> MPSATPGAPAASAAMQEALEGAGRIIDRLLQEDRAYPDLSELLNVPVHTCPTISGVSEMDYPLQSPGLLTIPSLPEISAIRRVPLPPELIEQFGHMQCNCMMGVFPEISRAWLTIDSDIFMWNYEDGGDLAYYDGLSETILSVGLVKPKTGIFQPHIRFLLVLSTPVDIVILGLSFANLQPGNLNDSISGGMQLLPDPLYSLPTDNTYLLSITSTDNGRIFLSGKDGCLYEVEYQAEAGWFSQRCRKINHSKSSLSFLVPSVLQFAFSEDDPIVQIAIDNSRNILYTRSEKGVIQVYDLGVDGHGMSRVASVSQNSLVSAAGNIARTIDRNVFKPIIHISVIEMSESVNCHLLAVTHTGVRFYFSTVPFKQPTARPCMLALVHVRLPPGFSASSNVEKPSKVHKALYNNGVLLMAASENEDNDMLWCINRDSFPFQKPMMETQVTTQVDGHSWALSAVDEQKADKIVTPLNKDLIPLTDSPVIIQQHMIPPKRFVLLSAQGSHIFYKLRPVDQLRHLLVSNSGGDGEEIERFFKLHQENQACATCLILACSSAASDREVSSWAARAFFRYGGEAQLRVQSALHAPSNVGPIFGSPLPVASPIPVGSPMPNPSFLGTPTQGACPPNVSTPAYGVATPAPQPPAVPGMMGTEIVFSGKHNGICIYFCRIIGNIWDGSVAVENTFQSGNREVTAIDSSVTPQHLESVLKELKGLLEFLDRYSQFTAGSLGNPGFGTPANRQQRLVSLGRPDIGSSQQAQQELQRKYHTEAQLAEQFSLQGIHQLVRKMCQALALWKLLCEHQFSLVVSDLQKELQEQLKITTFKDLVIRDKELTGALTASLISCYIRDNASVDGISYRLQEVCPLLYSTDDAVCSKANELLQRSRHVPNKQEKERMLRESLKEYQKISQQVDLPNVCAQYRQVRFYEGVVELCLSAAEKKDPQGLGLHFHKNGEPEEDMAGLQAFQERLNSYKCITDTLQELVNQSKAAPQSPSVPKKPGPPVLSSDPNMLSNEEAGIHFEQMLKLAQRSADELFNIALFNWLIQADLTDKLLELNSPFLEPHLVRMAKLDQNKVRYMDLLWRYYEKNRNFSNAARVVAKLADMHSPEISLKQRLEYISRAILSAKSSTTMSTLAADGEFLHELEEKLEVARIQL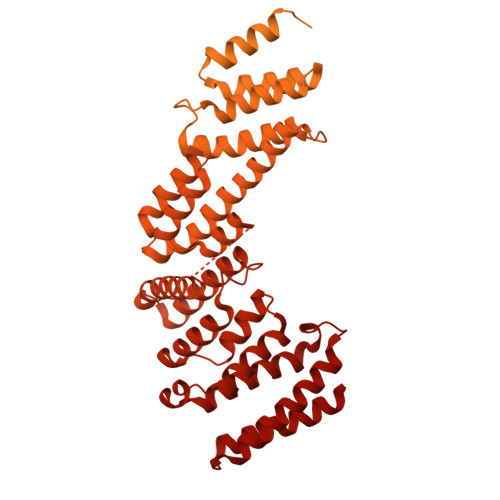QIQETLTRQYSHHSTVGDAVSQLDSQLMDITKMFGQYADPFRLSECKLAIIHCAGHSDPILVQTLWQDIIDKELSDSMGNSSVDRMQSLHLKITSLGKIYASTPRYFPLEFLVKYLEQQVCNFSWDAGFVTYTMQEINVPVPKLLEVYDHLFKARDPWWSRMKKPLHLLESIYILLSGYVQEPSKVPSYERRRFTTLCLDAISCYLVELQSMDPAPALLNTVSNFKSLQAKLERLS> AATTQIGEIVKTVANTVESEIKAELGVIPSLNAVETGATSNTEPEEAIQTRTVINMHGTAECLVENFLGRSALVCMRSFEYKNHSTSTSSIQKNFFIWTLNTRELVQIRRKMELFTYLRFDTEITIVPTLRLFSSSNVSFSGLPNLTLQAMYVPTGARKPSSQDSFEWQSACNPSVFFKINDPPARLTIPFMSINSAYANFYDGFAGFEKKATVLYGINPANTMGNLCLRVVNSYQPVQYTLTVRVYMKPKHIKAWAPRAPRTMPYTNILNNNYAGRSAAPNAPTAIVSHRSTIKTMPNDINLTTA;> SPSAEACGYSDRVLQLKLGNSSIVTQEAANICCAYGEWPTYLPDNEAVAIDKPTQPETSTDRFYTLKSKKWESNSTGWWWKLPDALNQIGMFGQNVQYHYLYRSGFLCHVQCNATKFHQGTLLIVAIPEHQIGKKGTGTSASFAEVMKGAEGGVFEQPYLLDDGTSLACALVYPHQWINLRTNNSATIVLPWMNSAPMDFALRHNNWTLAVIPVCPLAGGTGNTNTYVPITISIAP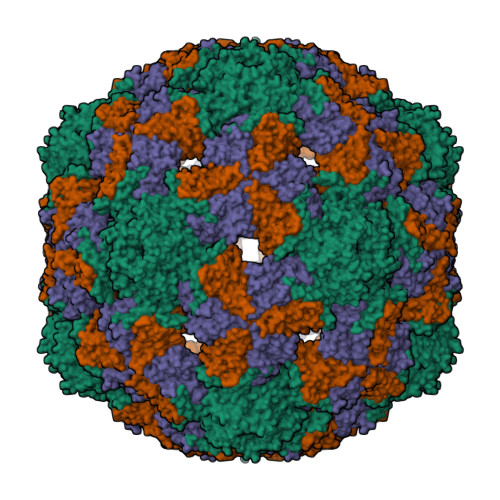MCAEYNGLRNAITQ;> GVPTCLLPGSNQFLTTDDHSSAPAFPDFSPTPEMHIPGQVHSMLEIVQIESMMEINNVNDASGVERLRVQISAQSDMDQLLFNIPLDIQLEGPLRNTLLGNISRYYTHWSGSLEMTFMFCGSFMTTGKLIICYTPPGGSSPTDRMQAMLATHVVWDFGLQSSITIIIPWISGSHYRMFNTDAKAINANVGYVTCFMQTNLVAPVGAADQCYIVGMVAAKKDFNLRLMRDSPDIGQSAILPEQ> PIETVPVKLKPGMDGPKVKQWPLTEEKIKALVEICTEMEKEGKISKIGPENPYNTPVFAIKKKDSTKWRKLVDFRELNKRTQDFWEVQLGIPHPAGLKKKKSVTVLDVGDAYFSVPLDEDFRKYTAFTIPSINNKTPGIRYQYNVLPQGWKGSPAIFQSSMTKILEPFRKQNPDIVIYQYMDDLYVGSDLEIGQHRTKIEELRQHLLRWGLTTPDKKHQKEPPFLWMGYELHPDKWTVQPIVLPEKDSWTVNDIQKLVGKLNWASQIYPGIKVRQLCKLLRG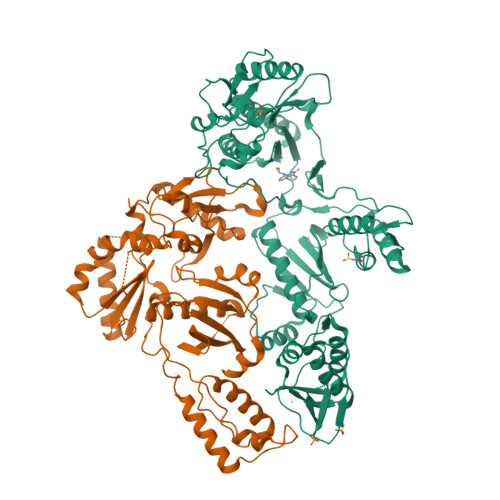TKALTEVIPLTEEAELELAENREILKEPVHGVYYDPSKDLIAEIQKQGQGQWTYQIYQEPFKNLKTGKYARMRGAHTNDVKQLTEAVQKITTESIVIWGKTPKFKLPIQKETWETWWTEYWQATWIPEWEFVNTPPLVKLWYQLEKEPIVGAETFYVDGAANRETKLGKAGYVTNRGRQKVVTLTDTTNQKTELQAIYLALQDSGLEVNIVTDSQYALGIIQAQPDQSESELVNQIIEQLIKKEKVYLAWVP;> TVPVKLKPGMDGPKVKQWPLTEEKIKALVEICTEMEKEGKISKIGPENPYNTPVFAIKKKDSTKWRKLVDFRELNKRTQDFWEVQLGIPHPAGLKKKKSVTVLDVGDAYFSVPLDEDFRKYTAFTIPSINNKTPGIRYQYNVLPQGWKGSPAIFQSSMTKILEPFRKQNPDIVIYQYMDDLYVGSDLEIGQHRTKIEELRQHLLRWGLTTPDKKHQKEPPFLWMGYELHPDKWTVQPIVLPEKDSWTVNDIQKLVGKLNWASQIYPGIKVRQLCKLLRGTKALTEVIPLTEEAELELAENREILKEPVHGVYYDPSKDLIAEIQKQGQGQWTYQIYQEPFKNLKTGKYARMRGAHTNDVKQLTEAVQKITTESIVIWGKTPKFKLPIQKETWETWWTEYWQATWIPEWEFVNTPPLVKLWYQ> MENTENSVDSKSIKNLEPKIIHGSESMDSGISLDNSYKMDYPEMGLCIIINNKNFHKSTGMTSRSGTDVDAANLRETFRNLKYEVRNKNDLTREEIVELMRDVSKEDHSKRSSFVCVLLSHGEEGIIFGTNGPVDLKK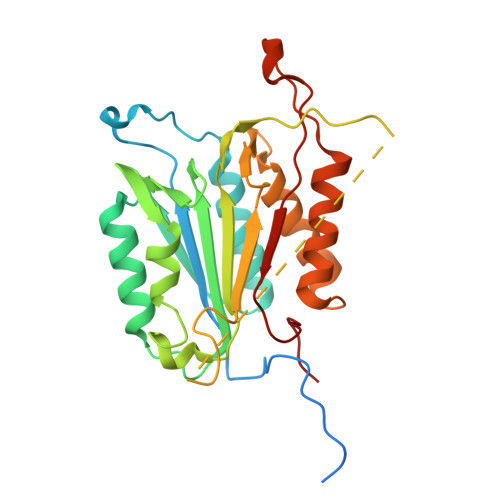ITNFFRGDRCRSLTGKPKLFIIQACRGTELDCGIETDSGVDDDMACHKIPVEADFLYAYSTAPGYYSWRNSKDGSWFIQSLCAMLKQYADKLEFMHILTRVNRKVATEFESFSFDATFHAKKQIPCINSMLTKELYFYHL> MGDEEKKEKKKKSKKKSEEEGGDAAPAPPPPKPPSQKRRAQRSGSNVFAMFTQHQVQEFKEAFQLIDQDKDGFISKNDIRATFDSLGRLCTEQELD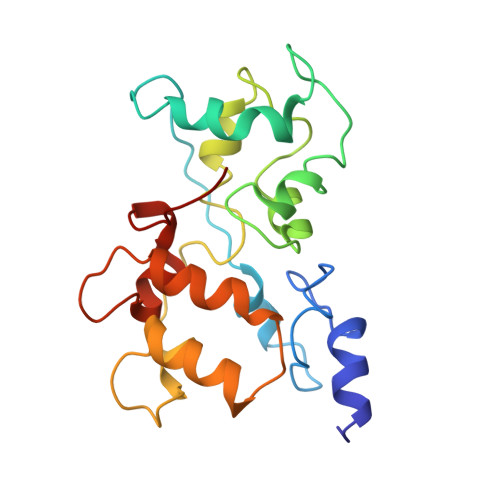SMVAEAPGPINFTMFLTIFGDRIAGTDEEDVIVNAFNLFDEGEGKCKEETLKRSLTTWGEKFSQDEVEEALSEAPIDGNGLIDIKKFAQILTKGAEEEGA N5-IMINOETHYL-L-ORNITHINE | 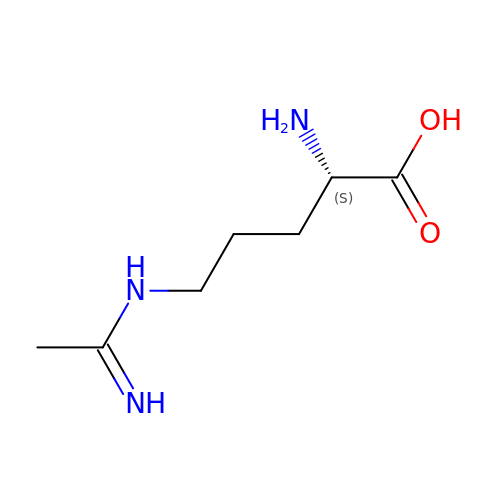C7 H15 N3 O2 | UYZFAUAYFLEHRC-LURJTMIESA-N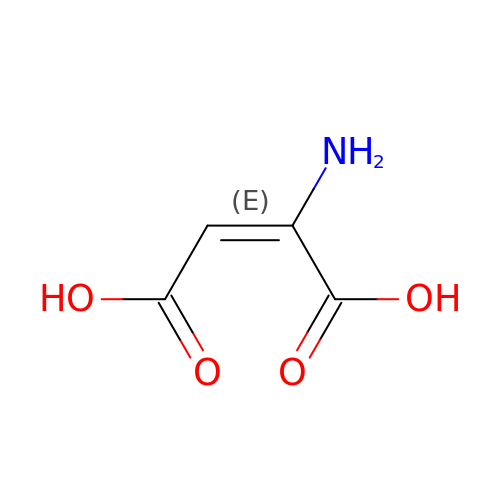2-amino maleic acid | C4 H5 N O4 | ABZHGLSYGDUSDL-OWOJBTEDSA-N>[2x]LGSSNDNIELVDFQNIMFYGDAEVGDNQQPFTFILDTGSANLWVPSVKCTTAGCLTKHLYDSSKSRTYEKDGTKVEMNYVSGTVSGFFSKDLVTVGNLSLPYKFIEVIDTNGFEPTYTASTFDGILGLGWKDLSIGSVDPIVVELKNQNKIENALFTFYLPVHDKHTGFLTIGGIEERFYEGPLTYE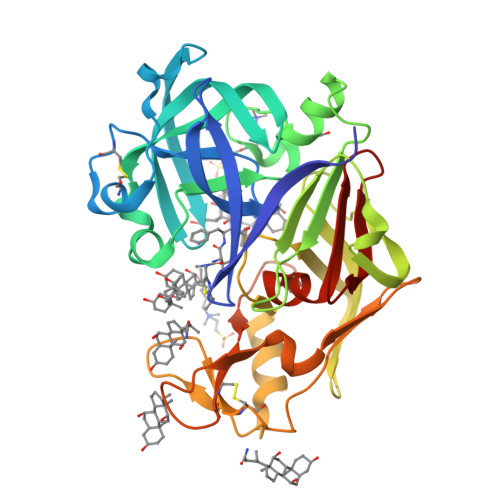KLNHDLYWQITLDAHVGNIMLEKANCIVDSGTSAITVPTDFLNKMLQNLDVIKVPFLPFYVTLCNNSKLPTFEFTSENGKYTLEPEYYLQHIEDVGPGLCMLNIIGLDFPVPTFILGDPFMRKYFTVFDYDNQSVGIALAKKNL> SMADRSPLHEAAAQGRLLALKTLIAQGVNVNLVTINRVSSLHEACLGGHVACAKALLENGAHVNGVTVHGATPLFNACCSGSAACVNVLLEFGAKAQLEVHLASPIHEAVKRGHRECMEILLANNVNIDHEVPQLGTPLYVACTYQRVDCVKKLLELGASVDHGQWLDTPLHAAARQSNVEVIHLLTDYGANLKRRNAQGKSAL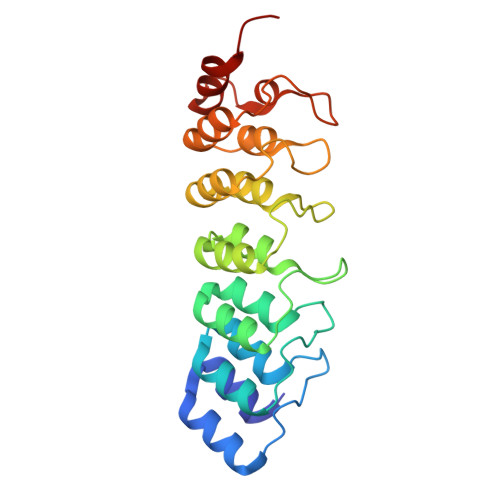DLAAPKSSVEQALLLREGPPAL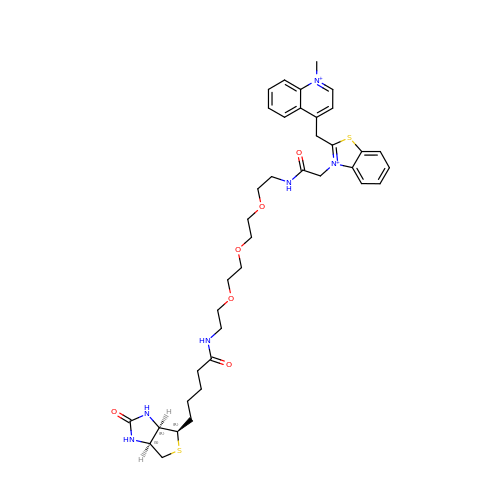4-[(3-{2,16-dioxo-20-[(3aR,4R,6aS)-2-oxohexahydro-1H-thieno[3,4-d]imidazol-4-yl]-6,9,12-trioxa-3,15-diazaicosan-1-yl}-1,3-benzothiazol-3-ium-2-yl)methyl]-1-methylquinolin-1-ium | C38 H50 N6 O6 S2 | SGYJIWSWMOUKKZ-GTCKRINLSA-P>KETAAAKFERQHMDSGGGGSGHMENGYTYEDYKNTAEWLLSHTKHRPQVAIICGSGLGGLTDKLTQAQIFDYGEIPNFPRSTVPGHAGRLVFGFLNGRACVMMQGRFHMYEGYPLWKVTFPVRVFHLLGVDTLVVTNAAGGLNPKFEVGDIMLIRDHINLPGFSGQNPLRGPNDERFGD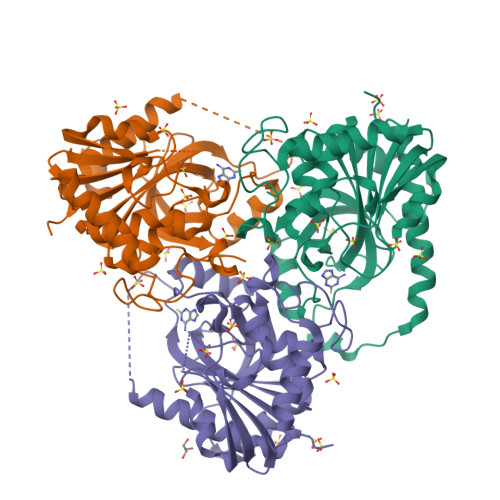RFPAMSDAYDRTMRQRALSTWKQMGEQRELQEGTYVMVAGPSFQTVAECRVLQKLGADAVGMSTVPEVIVARHCGLRVFGFSLITDKVIMDYESLEKANHEEVLAAGKQAAQKLEQFVSILMASIPLPDKAS[3x]>[2x]GPAMLTTRIIKETEKLQKECPPGITATPTKENPRYFMVTIQGPPQSCYEGGLFRLELFLPEEYPMKPPKVRFLTRIYHPNVDKVGRICLDIIKDKWSPALLINKVLLSIQILMSSPNPDDPLANDVAEHWKEDEASALQTAREWTRKYAKP;>GPAMVEVPRNFRLLEELETGEKGTGSNQNVSVGLRDTADIFFHYWNGTIVGPPSTTFEYRILSLEIYCDENYPKVPPHIRFLSKVNLPCVDSDGTVNREKFHVFKHWDRRTTMELCLSELRKEMAQPQNRKLVQPPEGSTY[2x]

We show that, amongst others, the E2 ubiquitin-conjugating enzyme UBC2 and the ubiquitin E2 variant UEV1 are essential for the promastigote to amastigote transition and subsequently characterise these proteins in biochemical and structural detail. We demonstrate that UBC2 and UEV1 form a heterodimer capable of carrying out ubiquitination and that the structural basis for this activity is conserved between Leishmania, Saccharomyces cerevisiae and humans. Therefore, L. mexicana UBC2 and UEV1 readily associate to form a heterodimeric UBC2-UEV1 complex. The UBC2-UEV1 heterodimer, like its S. cerevisiae and human orthologues, is able to form K63-linked ubiquitin chains in vitro, suggesting a role for non-degradative ubiquitin modifications in Leishmania differentiation.

Crystals, which appeared after two days from polyethylene glycol (PEG)-containing solutions, were sent for data collection at the Diamond Light Source, with the best crystal yielding a dataset extending to 1.7 Å spacing. Like its S. cerevisiae and human orthologues, UBC2 has a canonical E2 structure comprising a 4-stranded antiparallel β-sheet flanked by four α-helices. UEV1 exhibits a similar topology, but its polypeptide chain is shorter and the prominent pair of α-helices at the C-terminus of UBC2 (α3 and α4) are missing from UEV1. Superposing UBC2 with human UBE2N, UEV1 with human UBE2V2 or the UBC2-UEV1 and UBE2N-UBE2V2 heterodimers gives RMSDs of 0.82, 1.15 and 1.13 Å for 147, 135 and 271 equivalent atoms respectively, demonstrating a high level of structural conservation between these orthologues. The conserved active site residues, His75, Pro76, Asn77 and Cys85, reside on an extended segment of the polypeptide that connects strand β4 and helix α2 of UBC2, with the thiol group of Cys85 projecting out of the catalytic cleft. The interface between UBC2 and UEV1 involves the β2, β3 and β4 strands and the loops following β1, β3 and β4 of UBC2 and the N-terminus, α1 helix and loop following β1 of UEV1. The buried surface area of this interface is 1,466 Å2. The core of the interface contains a number of hydrophobic residues (Tyr32, Phe55, Leu70 and Val81 of UBC2 and Pro5, Phe8, Leu11, Leu14 and Phe39 of UEV1) that contribute strongly to the interaction. Hydrophobic residues are highly conserved at these positions, highlighting the importance of the associated hydrophobic interactions for complex formation. These hydrophobic interactions are complemented by a number of polar intermolecular interactions, mostly notably between the side chains of Glu53 of UBC2 and Asn7 of UEV1 and Arg68 of UBC2 and the main chain carbonyl oxygen of Ile37 of UEV1. Notably, a salt bridge is formed between Arg83 of UBC2 and Glu18 of UEV1.>GKAFDDGAFTGIRE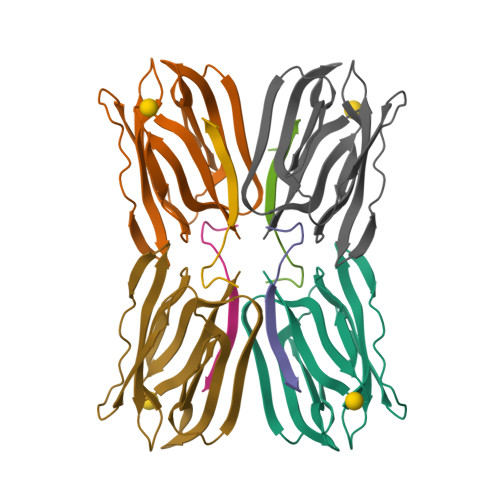INLSYNKETAIGDFQVVYDLNGSPYVGQNHVSFITGFTPVKISLDFPSEYIMEVSGYTGNVSGYVVVRSLTFKTNKKTYGPYGVTSGTPFNLPIENGLIVGFKGSIGYWLDYFSMYLSL[2x];>DEQSGISQTVIVGPWGAKSS[4x];>GKAFDDGAFTGIREINLSYNKETAIGDFQVVYDLNGSPYVGQNHKSFITGFTPVKISLDFPSEYIMEVSGYTGNVSGYVVVRSLTFKTNKKTYGPYGVTSGTPFNLPIENGLIVGFKGSIGYWLDYFSMYLSL[2x]> GSHTAEEDMEDDTSWRSEATFQFTVERFSRLSESVLSPPCFVRNLPWKIMVMPRFYPDRPHQKSVGFFLQCNAESDSTSWSCHAQAVLKIINYRDDEKSFSRRISHLFFHKENDWGFSNFMAWS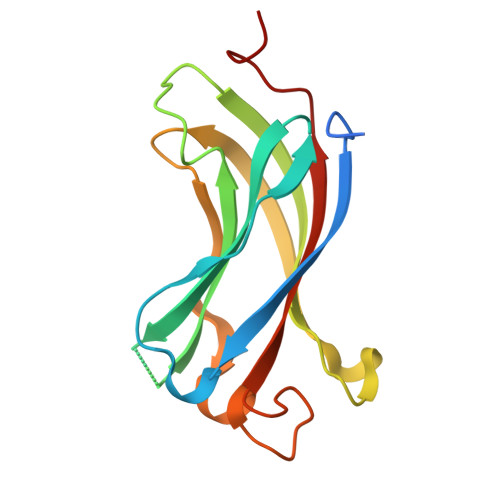EVTDPEKGFIDDDKVTFEVFVQADAPHGVAW>GSSPSLEQDDGDEETSVVIVGKISFCPKDVLGHGAEGTIVYRGMFDNRDVAVKRILPECFSFADREVQLLRESDEHPNVIRYFCTEKDRQFQYIAIELCAATLQEYVEQKDFAHLGLEPITLLQQTTSGLAHLHSLNIVHRDLKPHNILISMPNAHGKIKAMISDFGLCKKLAVGRHSFSRRSGVPGTEGWIAPEMLSEDCKENPTYTVDIFSAGCVFYYVISEGSHPFGKSLQRQANILLGACSLDCLHPEKHEDVIARELIEKMIAMDPQKRPSAKHVLKHPFFWSLEKQLQFFQDVS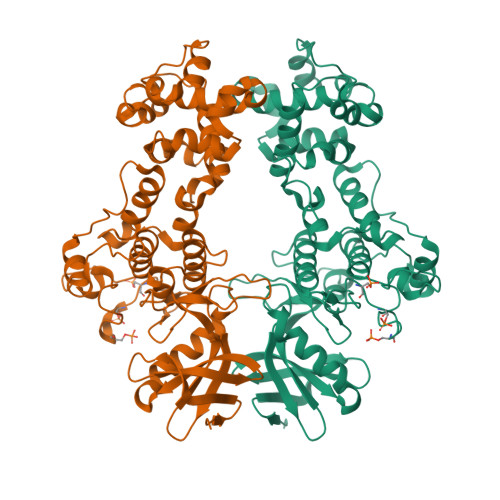DRIEKESLDGPIVKQLERGGRAVVKMDWRENITVPLQTDLRKFRTYKGGSVRDLLRAMRNKKHHYRELPAEVRETLGSLPDDFVCYFTSRFPHLLAHTYRAMELCSHERLFQPYYFHEPPEPQPPVTPDALGNS[4x]> IVGGYTCQENSVPYQVSLNSGYHFCGG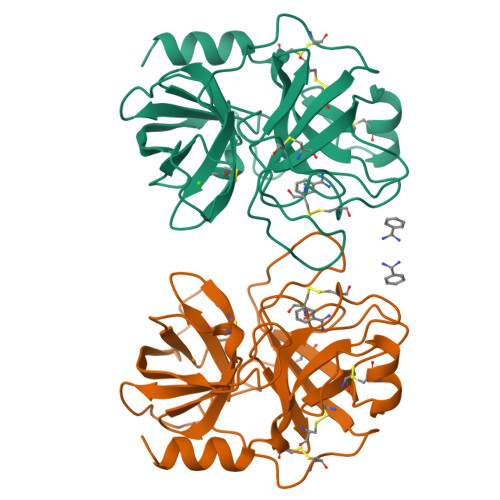SLINDQWVVSAAHCYKSRIQVRLGEHNINVLEGNEQFVNAAKIIKHPNFDRKTLNNDIMLIKLSSPVKLNARVATVALPSSCAPAGTQCLISGWGNTLSSGVNEPDLLQCLDAPLLPQADCEASYPGKITDNMVCVGFLEGGKDSCQGDSGGPVVCNGELQGIVEWGYGCALPDNPGVYTKVCNYVDWIQDTIAAN>[2x]ACPAPPPGQPDIRAIGYYTDKAGSVIDPALQQQNKDATAPLDRYAADVARMSDDYLRNGDPAAAQCTLSWLGAWADDGAMLGQMIRVNNDQSFYMRQWMLDAVAMAYLKVHDQANPQQRARIDPWLQKLARANLAYWDNPKRRRNNHYYWGGLGVLATGLATDDDALWQAGHAAFQKGIDDIQDDGSLPLEMARGQRALHYHDYALAPLVMMAELARLRGQDWYASRNHAIDRLARRVIEGSRDPAWFNQHTGAAQLPLQASGWVEFYRLRSPDGGVFDAAHARGPFHSPRLGGDLTLMATHGIVRTPLRHHHHHH

Unlike other PLs, Smlt1473 present in the clinically relevant Stenotrophomonas maltophilia strain K279a demonstrates a wide range of pH-dependent substrate specificities toward multiple, diverse polysaccharides: hyaluronic acid (pH 5.0), poly-β-D-glucuronic (celluronic) acid (pH 7.0), poly-β-D-mannuronic acid, and poly-α-L-guluronate (pH 9.0). To decode the pH-driven multiple substrate specificities and selectivity in this single enzyme, we present the X-ray structures of Smlt1473 determined at multiple pH values in apo and mannuronate-bound states as well as the tetra-hyaluronate-docked structure. We have built and refined the structures from residues A22-L330; electron density for other residues outside this range was either weak or absent. The structure is composed of 13 α-helical segments (α-1 to α-13) connected by 14 loops (L-1 to L-14) and two β-strands (β-1 and β-2) (Fig. 2, B and C (i and ii)).

To gain insight into this possibility, we analyzed the statistical distribution of B-factors in different apo structures at pH 5.0, 7.0, and 9.0, which were solved at comparable resolutions of 2.63, 2.20, and 2.45 Å, respectively. The protein is least flexible at acidic pH, most flexible at neutral pH, and has intermediate flexibility at basic pH. In particular, Smlt1473 has maximum activity for polyGlcA at pH 7.0 as well as the greatest spread in activity with regards to pH (>75% of maximum specific activity retained between pH 5.5 and pH 8.0) and also the largest observed B-factor. However, significant rotameric transitions of important substrate-binding residues such as K42, K162, R163, H221, and R312L have been observed at different pH values. At the entry site, the residues involved in rotameric transition are H221 and R312, of which H221 has an altered orientation in all structures above pH 5.0, whereas R312 has an altered orientation only in the pH 7.0 structure due to a hydrogen bonding interaction with Y225. Y38 and Y39 are part of the N-terminal lid loop constituting the R3 surface of the entry site, R218 constituting the roof R2 surface of the entry site, W171 and Y225 forming the iRW surface of the entry site, and R312 forming the F1 and F2 surface of the entry site. At the exit site (Fig. 8D (i)), the pH 7 apo structure has continuation of the high atomic fluctuations in the same left side from the exit site view (i LW and ii LW surface) and includes residues such as K42, Y115, H168, and R215. We found that pH 5.0, 7.0, and 9.0 have, respectively, two (N55, Y222), four (Y38, Q112, N167, H168), and three (R215, R218, H221) residues with the highest atomic fluctuations at the [−1, +1] subsite. This generalization implicates the pH 7.0 apo structure catalytic tunnel to be the most flexible and rationalizes the less numerous and weaker interactions for the ManA cocrystallized pH 7.0 structure compared with pH 5.0, as discussed in the previous section.N-[([1,1'-biphenyl]-4-yl)methyl]-N-[4-(1,1,1,3,3,3-hexafluoro-2-hydroxypropan-2-yl)phenyl]benzenesulfonamide | C28 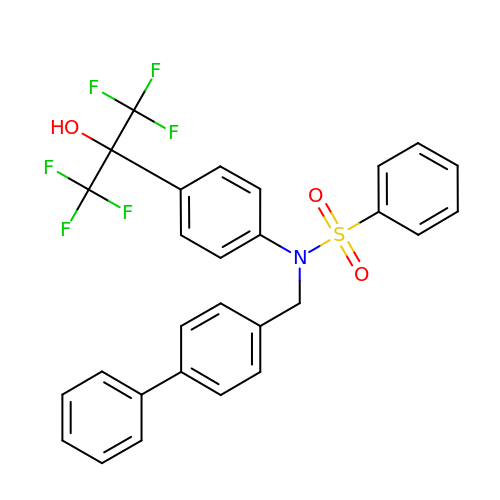H21 F6 N O3 S | QNAWYCWKQPMYME-UHFFFAOYSA-N> TGGRNSIRYSELAPLFDTTRVYLVDNKSTDVASLNYQNDHSNFLTTVIQNNDYSPGEASTQTINLDDRSHWGGDLKTILHTNMPNVNEFMFTNKFKARVMVSRSLTKDKQVELKYEWVEFTLPEGNYSET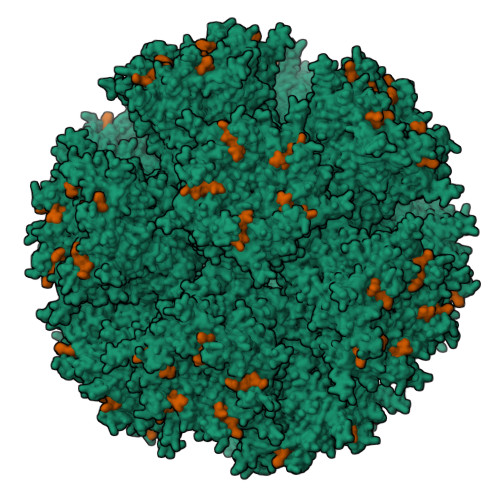MTIDLMNNAIVEHYLKVGRQNGVLESDIGVKFDTRNFRLGFDPVTGLVMPGVYTNEAFHPDIILLPGCGVDFTHSRLSNLLGIRKRQPFQEGFRITYDDLEGGNIPALLDVDAYQASLKDDTEQGGDGAGGGNNSGSGAEENSNAAAAAMQPVEDMNDHAIRGDTFATRAEEKRAEAEAAAEAAAPAAQPEVEKPQKKPVIKPLTEDSKKRSYNLISNDSTFTQYRSWYLAYNYGDPQTGIRSWTLLCTPDVTCGSEQVYWSLPDMMQDPVTFRSTSQISNFPVVGAELLPVHSKSFYNDQAVYSQLIRQFTSLTHVFNRFPENQILARPPAPTITTVSENVPALTDHGTLPLRNSIGGVQRVTITDARRRTCPYVYKALGIVSPRVLSSRTF;> MKRARPSEDTFNPVYPYDTEC A single ER‐localised Fic protein, FICD (HYPE), catalyses both AMPylation and deAMPylation of BiP. FICD is a class II Fic protein (with its αinh N‐terminal to its Fic domain) and an ER‐localised type II, single‐pass transmembrane protein, with a short cytoplasmic portion and a large luminal‐facing catalytic domain (Worby et al, 2009; Bunney et al, 2014). We report on the transition of FICD from a dimeric enzyme, that deAMPylates BiP, to a monomer with potent AMPylation activity. Mechanistically, monomerisation relieves a repressive effect allosterically propagated from the dimer interface to the inhibitory Glu234, thereby permitting AMPylation‐competent binding of MgATP.

The crystal structure of dimeric FICD suggests the existence of a hydrogen‐bond network, involving the side chains of Lys256 and Glu242, linking the dimer interface with the enzyme's active site, impinging on the AMPylation‐inhibiting Glu234. Mutation of the dimer relay residue Lys256 does not result in large conformational changes in FICD. (ii) The dimeric dimer relay mutant FICDK256A displays a clear MgATP density up to and including the γ‐phosphate phosphorous atom. As noted in other Fic AMPylases, this Mg2+ was coordinated by the α‐ and β‐phosphates of ATP/AMPPNP and Asp367 of the Fic motif (Xiao et al, 2010; Bunney et al, 2014; Khater & Mohanty, 2015b). By contrast, in the active sites of FICDK256A or FICDL258D MgATP and MgAMPPNP assumed AMPylation‐competent conformations: their α‐phosphates were in the canonical position (Fig EV4E), as defined by AMPylation‐active Fic proteins lacking inhibitory glutamates (Xiao et al, 2010; Engel et al, 2012; Goepfert et al, 2013; Bunney et al, 2014). As a result, in‐line nucleophilic attack into the α‐β‐phosphoanhydride bond of ATP would not be sterically hindered and the Nε2 of His363 would be well positioned for general base catalysis (and EV4C and D). Concordantly, the RMSD of ATP between the wild‐type FICD and monomeric FICDL258D was 2.17 Å (and 2.23 Å for FICDK256A's ATP). The disparities in the manner of FICD‐ATP binding are well explained by a monomerisation‐induced increase in Glu234 flexibility (mediated by weakening of the dimer relay), as reflected in the lower melting temperatures of FICDK256A and FICDL258D relative to the wild‐type dimer and localised B‐factor increases in their respective crystal structures.

> SLEARAALNQALEMKRQGKREKAQKLFMHALKMDPDFVDALTEFGIFSEEDKDIIQADYLYTRALTISPYHEKALVNRDRTLPLVEEIDQRYFSIIDSKVKKVMSIPKGNSALRRVMEETYYHHIYHTVAIEGNTLTLSEIRHILETRYAVPGASLEEQNEVIGMHAAMKYINTTLVSRIGSVTISDVLEIHRRVLGYVDPVEAGRFRTTQVLVGHHIPPHPQDVEKQMQEFVQWLNSEEAMNLHPVEFAALAHYKLVYIHPFIDGNGRTSRLLMNLILMQAGYPPITIRKEQRSDYYHVLEAANEGDVRPFIRFIAKCTETTLDTLLFATTEYSVALPEAQP> ADTIVAVELDTYPNTDIGDPDYPHIGIDIKSVRSKKTAKWNMQNGKVGTAHIIYNSV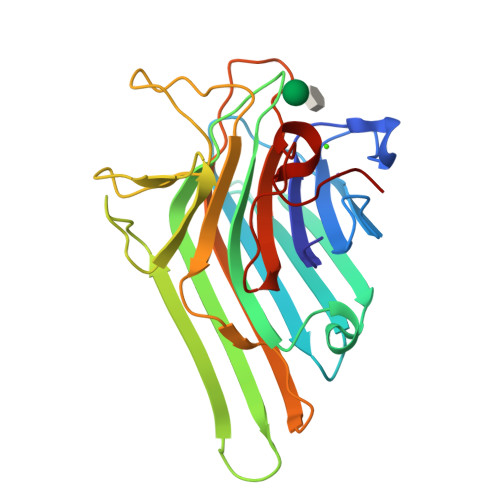GKRLSAVVSYPNGDSATVSYDVDLDNVLPEWVRVGLSASTGLYKETNTILSWSFTSKLKSNSTHETNALHFMFNQFSKDQKDLILQGDATTGTDGNLELTRVSSNGSPQGSSVGRALFYAPVHIWESSAVVASFDATFTFLIKSPDSHPADGIAFFISNIDSSIPSGSTGRLLGLFPDAN> SAETQMERKIIDFLRQNGKSIALTIAKEIGLDKSTVNRHLYNLQRSNQVFNSNEKPPVWDLM

Since these orthologs contain two left-handed deoxyribonucleic acid (Z-DNA) binding domains (ZBDs) instead of dsRBD of PKR, they were named as protein kinases containing ZBDs (PKZ). Therefore, PKZ is a functional ortholog of PKR but it recognizes Z-DNA instead of dsRNA. Zα domains commonly have a winged helix-turn-helix (wHTH) DNA binding motif and recognize Z-DNA in a conformation-specific manner. However, PKZ works as an innate immune sensor by recognizing poly-d(GC) as Z-DNA and turning off general translation machinery by phosphorylating eukaryotic translation initiation factor 2α (eIF2α).

To understand the difference in the B-to-Z transition rates of Zα domains in relation to their Z-DNA binding modes, we determined the crystal structure of caZαPKZ in complex with dsdT(dCdG)3 oligonucleotide at 1.7-Å resolution with R factor of 17.2% and Rfree of 22.6%. By the C2 symmetry operation, two caZαPKZ molecules bound to both sides of the Z-DNA in a head-to-tail orientation were generated. The overall structure of caZαPKZ is well conserved with three β strands and three α helices, like other members of the Zα family. In the complex structure, dsDNA molecules generated by the C2 symmetry operation adopt a canonical left-handed Z-DNA conformation. Interestingly, one manganese ion is coordinated with the backbone phosphate (P0), N7 of guanine 2 (G2) and four water molecules with an octahedral coordination geometry. The interaction between caZαPKZ and Z-DNA is mediated by five residues in the α3 core and four residues in the β-wing. Among them, Lys34, Asn38 and Arg39 in the α3 core form direct or water-mediated hydrogen bonds with backbone phosphates of Z-DNA, as observed in the hZαADAR1 structure. Tyr42, which is known as the most critical residue for Z-DNA binding by forming the CH−π stacking with the guanine 4 (G4), is conserved in structural and sequential aspects. Due to the shorter length and lack of positive charge, Ser35 does not form ionic interactions, but does have hydrogen bonding with the P3 phosphate.>GNSDDARTSIEQRSNAVSQVLLGIFSYVRWPKEPAVLQLCVVGPTEYADGLLRGMVQANGRRVHAERRAVDNPDLGTLSNVIYLGVVDERERQQVFRSLAGHPVLSISERGTECSVGSMFCLNVGGPRITFEANLDSIARSGVRVHPSVLKLARRQ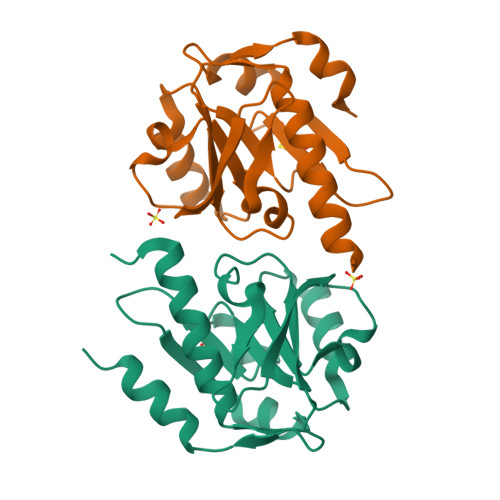ATP[2x]>[8x]MVWLANPERYGQMQYRYCGKSGLRLPALSLGLWHNFGHVNALESQRAILRKAFDLGITHFDLANNYGPPPGSAEENFGRLLREDFAAYRDELIISTKAGYDMWPGPYGSGGSRKYLLASLDQSLKRMGLEYVDIFYSHRVDENTPMEETASALAHAVQSGKALYVGISSYSPERTQKMVE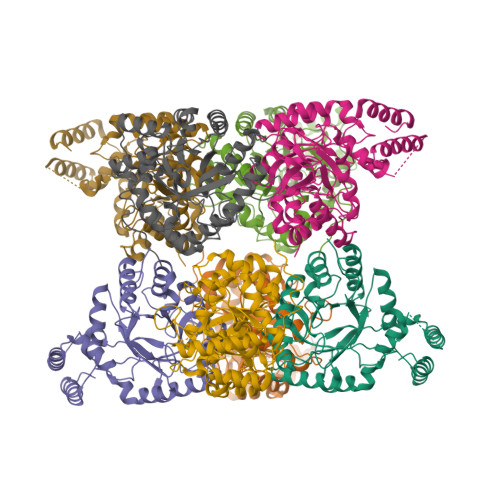LLREWKIPLLIHQPSYNLLNRWVDKSGLLDTLQNNGVGCIAFTPLAQGLLTGKYLNGIPQDSRMHREGNKVRGLTPKMLTEANLNSLRLLNEMAQQRGQSMAQMALSWLLKDDRVTSVLIGASRAEQLEENVQALNNLTFSTKELAQIDQHIADGELNLWQASSDK>MHHHHHHTMAAPVSTQLSQDELKKQAAWKAVEYVKSGMVVGLGTGSTAAFAVDRIGQLLKEGKLQNIVGVPTSIRTYEQALSLGIPLATLDEQPKLDVAIDGADEVDPNLDVVKGRGGALLREKMVEMASAKFVCIVDDSKLVEGLGGSKLAMPVEIVQFCHKYTLQRLANLPEVKGCEAKLRMNGDKPYVTDNSNYIVDLYFQTPIKDSQAASKAILGLDGVVDHGLFLDMVDVCIIAGATGVTVQERPNPKKH[2x]

Prior to this phosphorylation step, ribose-5-phosphate (R5P) carbonyl group is transferred from carbon 1 to carbon 2. This reaction is catalyzed by the metabolic enzyme ribose-5-phosphate isomerase (RPI). Beside its critical role in the CBC, RPIA is implicated in the non-oxidative branch of the pentose phosphate pathway (PPP). We describe the first structure of a ribose-5-phosphate isomerase from a Viridiplanta, the model microalga Chlamydomonas reinhardtii. The structural fold of CrRPI1 is similar to previously described structures of canonical RPIA even though plastidial RPI participates in both the Calvin-Benson cycle and the pentose phosphate pathway.

We solved the crystal structure of CrRPI1 in the P21 space group at 1.40 Å resolution. Each monomer is composed of six alpha helices and twelve beta strands distributed into two domains. The first domain contains the catalytic pocket, while the second was proposed to play a role in the oligomerization of RPIA. CrRPI1 is a homodimer in solution and in the crystal packing. The homodimeric state is also observed in the crystal asymmetric unit with α helices h4, h5 and h6 and β strands s10 contributing to the interface. CrRPI1 catalytic site is described free from substrate and product, representing the apo state of the enzyme. Six water molecules, a sulfate ion and a sodium ion are however present and therefore allow to predict the coordination and placement of its substrate R5P in this pocket through structural superposition and sequence analysis. The sulfate ion in CrRPI1 hence occupies the location of the phosphate of the ribose-5-phosphate supporting a conserved mode of substrate recognition. This sulfate ion is coordinated by polar contacts with the side chains of S60, T61, and K155 and the main chain amine of T61. In our CrRPI1 crystal structure, C149 and C250 position their sulfur atoms 4.4 Å apart, a distance compatible with the formation of a disulfide bridge.>[4x]GPHMLEAEHPLQYNYTFWYSRRTPGRPTSSQSYEQNIKQIGTFASVEQFWRFYSHMVRPGDLTGHSDFHLFKEGIKPMWEDDANK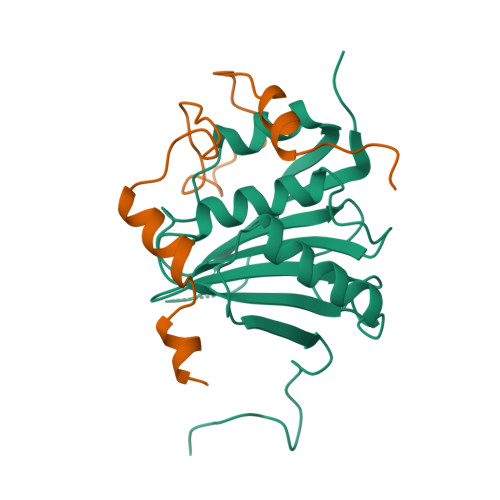NGGKWIIRLRKGLASRCWENLILAMLGEQFMVGEEICGAVVSVRFQEDIISIWNKTASDQATTARIRDTLRRVLNLPPNTIMEYKTHTDSIKMPGRLGPQRLLF;>[4x]GPHMKYKLADYRYGREEMLALYVKENKVPEELQDKEFAAVLQDEPLQPLALEPLTEEEQRNFSLSVNSVAVLRLM>GSNRTLIVTTILEEPYVMYRKSDKPLYGNDRFEGYCLDLLKELSNILGFLYDVKLVPDGKYGAQNDKGEWNGMVKELIDHRADLAVAPLTITYVREKVIDFSKPFMTLGISILYRKGTPIDSADDLAKQTKIEYGAVRDGSTMTFFKKSKISTYEKMWAFMSSRQQSALVKNSDEGIQR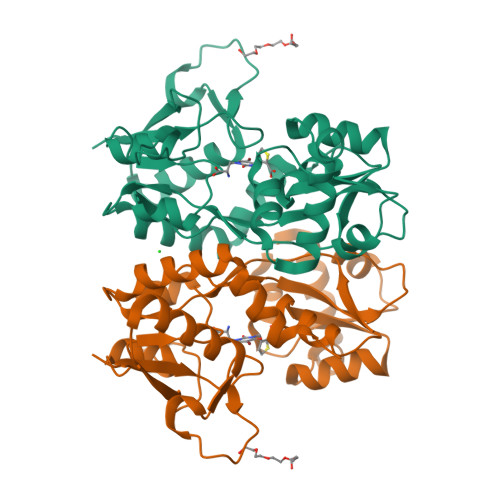VLTTDYALLMESTSIEYVTQRNCNLTQIGGLIDSKGYGVGTPIGSPYRDKITIAILQLQEEGKLHMMKEKWWRGNGCPS[2x]> MLGGLLHRGHKIKGTVVLMRKNVLDVNSVTSVGGIIGQGLDLVGSTLDTLTAFLGRSVSLQLISATKADANGKGKLGKATFLEGIITSLPTLGAGQSAFKINFEWDDGSGIPGAFYIKNFMQTEFFLVSLTLEDIPNHGSIHFVCNSWIYNAKLFKSDRIFFANQTYLPSETPAPLVKYREEELHNLRGDGTGERKEWERIYDYDVYNDLGDPDKGENHARPVLGGNDTFPYPRRGRTGRKPTRKDPNSESRSNDVYLPRDEAFGHLKSSDFLTYGLKSVSQNVLPLLQSAFDLNFTPREFDSFDEVHGLYSGGIKLPTDIISKISPLPVLKEIFRTDGEQALKFPPPKVIQVSKSAWMTDEEFAREMLAGVNPNLIRCLKDFPPRSKLDSQVYGDHTSQITKEHLEPNLEGLTVDEAIQNKRLFLLDHHDP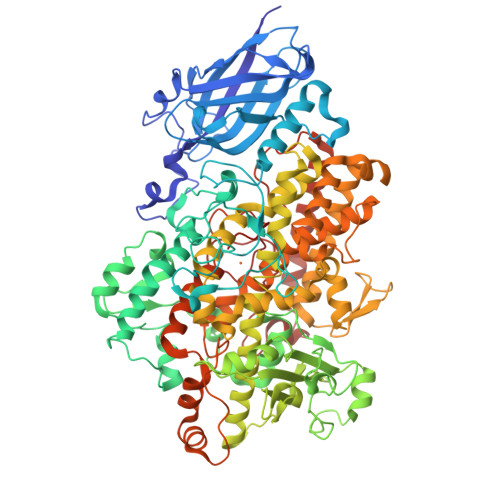IMPYLRRINATSTKAYATRTILFLKNDGTLRPLAIELSLPHPQGDQSGAFSQVFLPADEGVESSIWLLAKAYVVVNDSCYHQLVSHWLNTHAVVEPFIIATNRHLSVVHPIYKLLHPHYRDTMNINGLARLSLVNDGGVIEQTFLWGRYSVEMSAVVYKDWVFTDQALPADLIKRGMAIEDPSCPHGIRLVIEDYPYTVDGLEIWDAIKTWVHEYVFLYYKSDDTLREDPELQACWKELVEVGHGDKKNEPWWPKMQTREELVEACAIIIWTASALHAAVNFGQYPYGGLILNRPTLSRRFMPEKGSAEYEELRKNPQKAYLKTITPKFQTLIDLSVIEILSRHASDEVYLGERDNPNWTSDTRALEAFKRFGNKLAQIENKLSERNNDEKLRNRCGPVQMPYTLLLPSSKEGLTFRGIPNSISI> MRIEVIRREENLLEFYLEGEDHTFANLLTETLHE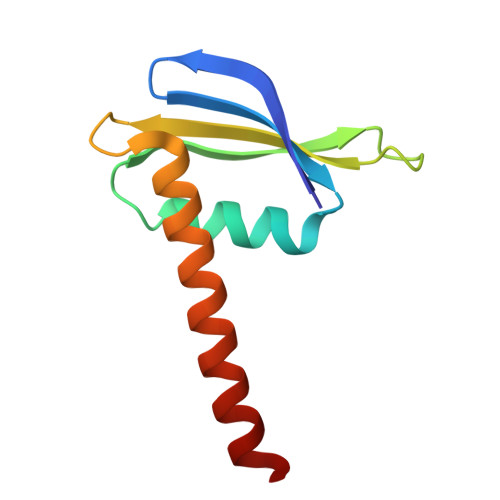NEHVTFAGYTIEHPITMARKPRFKVVTDGKITPEKALEEAAQKIFDRAREVLEAWKAAIE>GSHMVKVQVKQLQGMSLTRKVHPSTTVWELKGEIEKEWCIPRYQQRLALQDNPSNLPALRDGDSLAAHGLFYDIVLLLLCTEPQEMEVLVKDSNKTTVYTVRPTDTVKQLKQQIYACQHVPVEQQRLTYETKELENHHTLEHYHVQPRSTIYL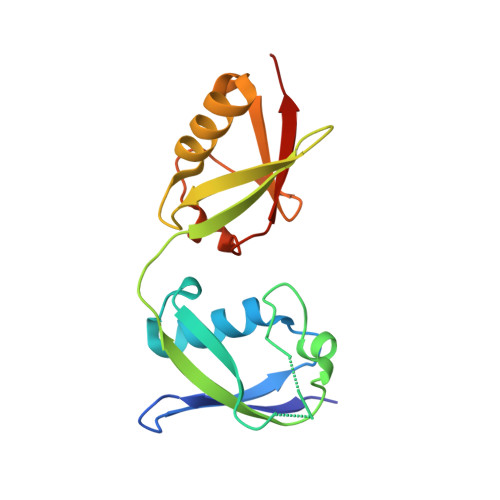LLRLRGG[2x]>MDRLDFSIKLLRKVGHLLMIHWGRVDNVEKKTGFK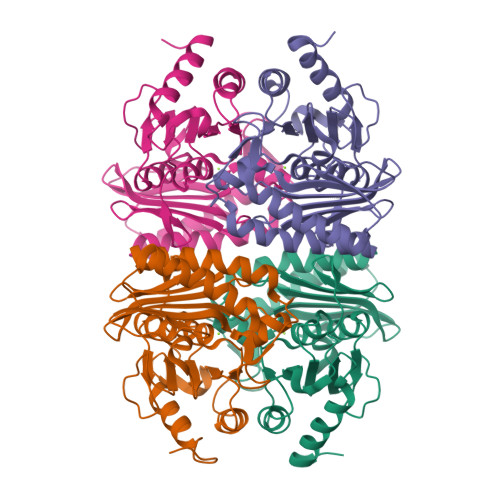DIVTEIDREAQRMIVDEIRKFFPDENIMAEEGIFEKGDRLWIIDPIDGTINFVHGLPNFSISLAYVENGEVKLGVVHAPALNETLYAEEGSGAFFNGERIRVSENASLEECVGSTGSYVDFTGKFIERMEKRTRRIRILGSAALNAAYVGAGRVDFFVTWRINPWDIAAGLIIVKEAGGMVTDFSGKEANAFSKNFIFSNGLIHDEVVKVVNEVVEEIGGK[4x]The Rho factor is a ring-shaped ATP-dependent hexameric helicase that is conserved throughout the bacterial kingdom. Rho plays an indispensable function in transcriptional termination and gene regulation in bacteria. Rof (Rho-off, also called YaeO) is the only E. coli host factor that directly interacts with Rho and inhibits the Rho-dependent transcription termination. Rof binds to the open-ring Rho hexamer and inhibits the initiation of Rho-dependent termination.

The assembled complex was further validated in gel filtration assay, and the results confirmed the extensive interactions between Rof and Rho. We subjected the assembled complex to single-particle reconstruction cryo-EM study and determined a 2.8 Å resolution structure of the Rho-Rof complex. The overall structure shows a Rho hexamer (open-ring state, comprising six protomers A-F) interacting with six Rof proteins in each of its protomers. The architecture of Rho is identical to previously reported open-ring state Rho structures, in which the midpoints of protomers A and F at either end of the ring are offset by 45 Å and leaves a 12 Å wide gap. Rof binds extensively to Rho by attaching its N-terminal α-helix to the N-terminal of Rho. The negative-charged residues Asn9, Asp11, Asp14 from Rof N-terminal α-helix form hydrogen bonds and salt bridges with Lys115, Lys105, Ser82, Gln85, Ser84 in Rho, respectively. In addition, residues Cys10 and Tyr13 stabilize the interface via van der Waals interactions with residues Leu114, Phe 89. The Rof’s β3-β4 loops (residues 45–50) make additional interactions with two Rho protomers. As showed in Fig. 1d, the residues Arg46, Lys47, Asn48, and Glu50 from β3-β4 loops make contacts with both protomer D and C by forming strong hydrogen bonds with residues Gly22, Glu19, Glu125, and Arg88, respectively. It appears that the open-ring gap between protomer F and A is causing a disruption in the interactions between Rof’s β3-β4 loops and Rho. As a result, the density of Rof in protomer F is considerably worse and has lower local resolution compared to the other protomers of Rho.

>MNLTELKNTPVSELITLGENMGLENLARMRKQDIIFAILKQHAKSGEDIFGDGVLEILQDGFGFLRSADSSYLAGPDDIYVSPSQIRRFNLRTGDTISGKIRPPKEGERYFALLKVNEVNFDKPENARNKILFENLTPLHANSRLRMERGNGSTEDLTARVLDLASPIGRGQRGLIVAPPKAGKTMLLQNIAQSIAYNHPDCVLMVLLIDERPEEVTEMQRLVKGEVVASTFDEPASRHVQVAEMVIEKAKRLVEHKKDVIILLDSITRLARAYNTVVPASGKVLTGGVDANALHRPKRFFGAARNVEEGGSLTIIATALIDTGSKMDEVIYEEFKGTGNMELHLSRKIAEKRVFPAIDYNRSGTRKEELLTTQEELQKMWILRKIIHPMGEIDAMEFLINKLAMTKTNDDFFEMMKRS[6x];>[6x]MNDTYQPINCDDYDNLELACQHHLMLTLELKDGEKLQAKASDLVSRKNVEYLVVEAAGETRELRLDKITSFSHPEIGTVVVSES>AGNFELEILEISNTNSHLLNGYCCGMPAELRATKTIGCSPCTTAFRLCLKEYQTTEQGASISTGCSFGNATTKILGGSSFVLSDPGVGAIVLPFTFRWTKSFTLILQALDMYNTSYPDAERLIEETSYSGVILPSPEWKTLDHIGRNARITYRVRVQCAVTYYNTTCTTFCRPRDDQFGHYACGSEGQKLCLNGWQGVNCEEAICKAGCDPVHGKCDRPGECECRPGWRGPLCNECMVYPGCKHGS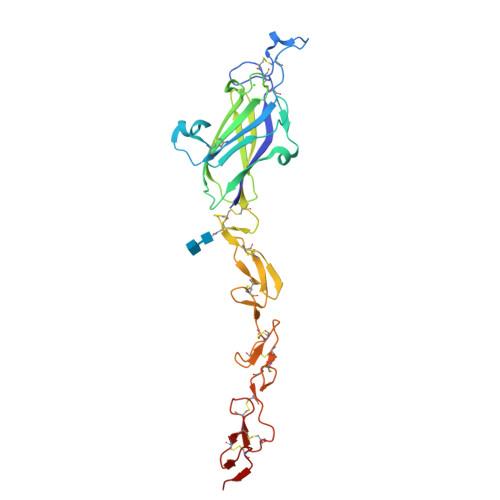CNGSAWKCVCDTNWGGILCDQDLN[2x]(1R)-2-(phosphonooxy)-1-[(tridecanoyloxy)methyl]ethyl pentadecanoate | C31 H61 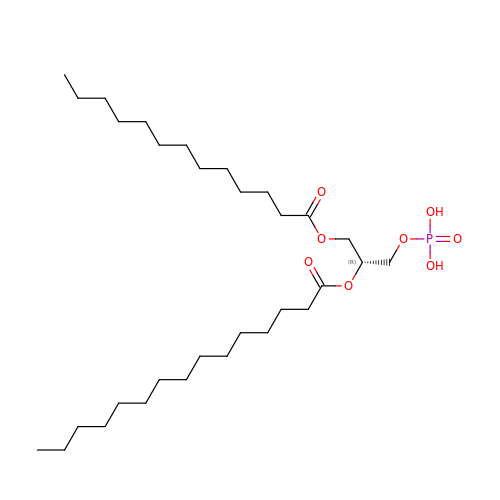O8 P | UOOPRMYYAWVCCZ-GDLZYMKVSA-N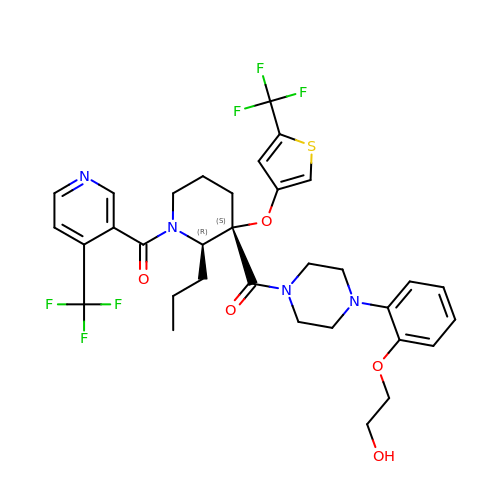{4-[2-(2-hydroxyethoxy)phenyl]piperazin-1-yl}[(2R,3S)-2-propyl-1-{[4-(trifluoromethyl)pyridin-3-yl]carbonyl}-3-{[5-(trifluoromethyl)thiophen-3-yl]oxy}piperidin-3-yl]methanone | C33 H36 F6 N4 O5 S | KEKDAGVCTZPOAA-JOMNFKBKSA-N3-(2-{1-[2-(piperidin-4-yl)ethyl]-1H-indol-5-yl}-5-[1-(pyrrolidin-1-yl)cyclohexyl]-1,3-thiazol-4-yl)-N-(2,2,2-trifluoroethyl)prop-2-yn-1-amine 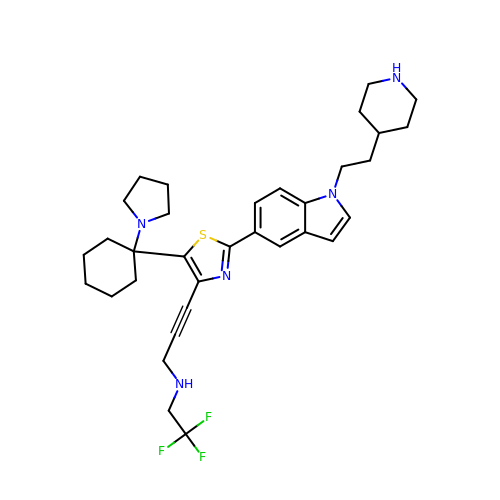| C33 H42 F3 N5 S | RQISOXZUFXHDIM-UHFFFAOYSA-N> VADRYAVYWNSSNPRFQRGDYHIDVCINDYLDVFCPHYEDSVPEDKTERYVLYMVNFDGYSACDHTSKGFKRWECNRPHSPNGPLKFSEKF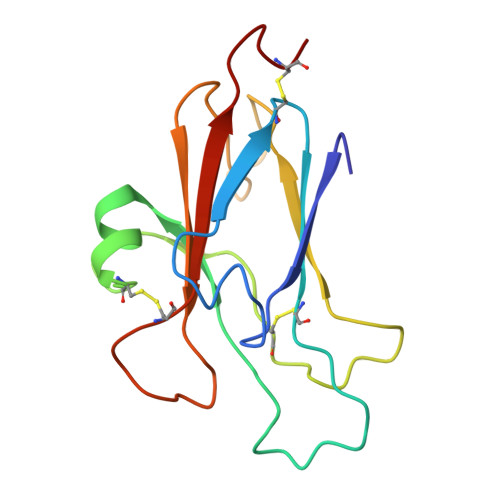QLFTPFSLGFEFRPGREYFYISSAIPDNGRRSCLKLKVFVRPTNSCM6-CHLORO-4-(CYCLOHEXYLOXY)-3-PROPYLQUINOLIN-2(1H)-ONE | C18 H22 Cl N O2 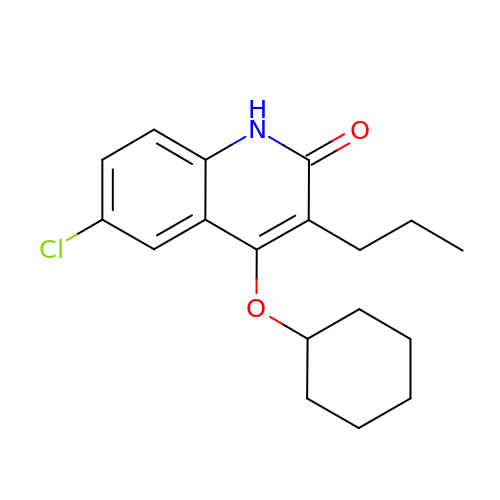| BNZHKKGOSYAQSW-UHFFFAOYSA-N>[2x]SALAQQLPGTWKMDVTSEDGVRTTGQMHIQPKTP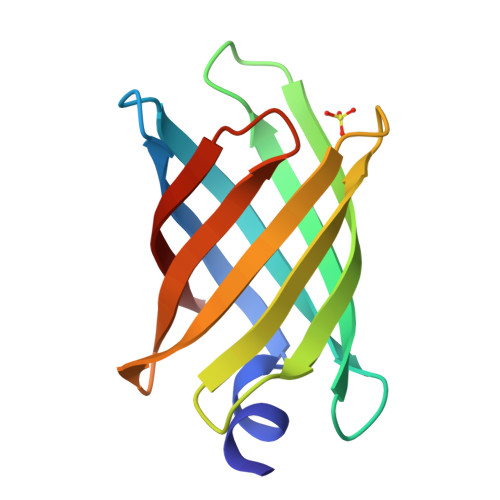TTMDVTLTGTHADGKPFTGQGKITVKTPTTVDITVTYEDGSTATGQLTVDSPTQFKFDMTASDGTRFTGTVQRQS> XQVPELIKPS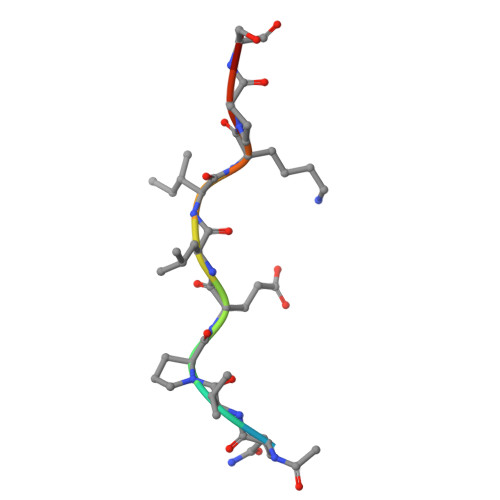Q>[2x]GSKEKLKEIKLLVCNIDGCLTNGHIYVSGDQKEIISYDVKDAIGISLLKKSGIEVRLISERACSKQTLSALKLDCKTEVSVSDKLATVDEWRKEMGLCWKEVAYLGNEVSDEECLKR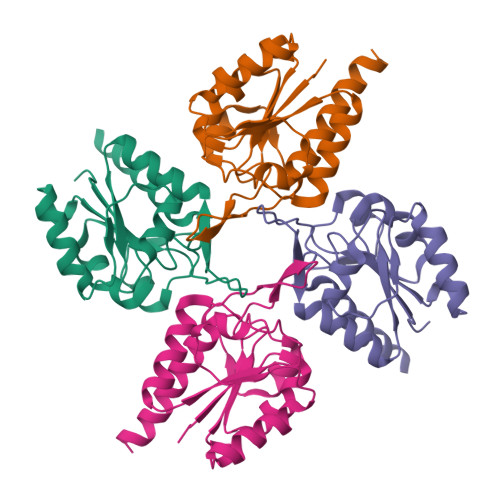VGLSAVPADACSGAQKAVGYICKCSGGRGAIREFAEHIFLLIEKVNNSCQK>GSHMSVVGTPKSAEQIQQEWDTNPRWKDVTRTYSAEDVVALQGSVVEEHTLARRGAEVLWEQLHDLEWVNALGALTGNMAVQQVRAGLKAIYLSGWQVAGDANLSGHTYPDQSLYPANSVPQVVRRINNALQRADQIAKIEGDTSVENWLAPIVADGEAGFGGALNVYELQKALIAAGVAGSHWEDQLASEKKCGHLGGKVLIPTQQHIRTLTSARLAADVADVPTVVIARTDAEAATLITSDVDERDQPFITGERTREGFYRTKNGIEPCIARAKAYAPFADLIWMETGTPDLEAARQFSEAVKAEYPDQMLAYNCSPSFNWKKHLDDATIAKFQKELAAMGFKFQFITLAGFHALNYSMFDLAYGYAQNQMS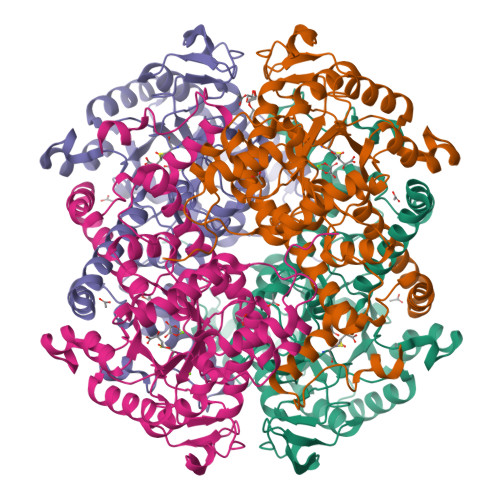AYVELQEREFAAEERGYTATKHQREVGAGYFDRIATTVDPNSSTTALTGSTEEGQFH[4x]>[2x]TRRTAFFFDELCLWHAAGPHALTLPVGGWVQPPAAAGHAESPETKRRLKSLLDVSGLTARLQLRSAPPASDEDLLRVHPAHYLERFKALSDAGGGSLGQDAPIGPGSYEIARLSAGLAIAALDAVLAGEADNAYSLSRPPGHHCLPDQAMGFCFFANIAVAIEAAKARHGVERVAVLDWDVHHGNGT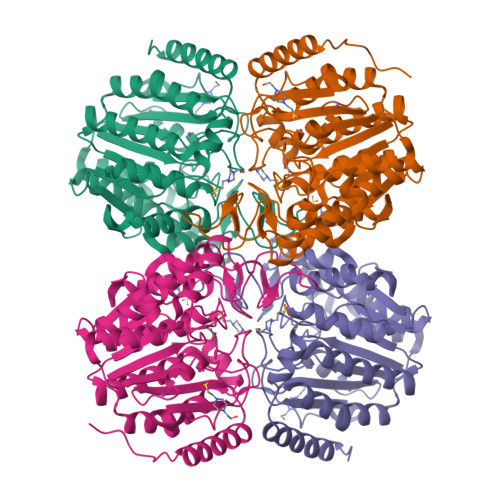QAIYYRRDDVLSISLHQDGCFPPGYSGAEDIGEDRGRGFNLNVPLLPGGGHDAYMQAMQRIVLPALERFRPQLIVVASGFDANAVDPLARMQLHSDSFRAMTAMVRDAAERHAGGRLVVVHEGGYSEAYVPFCGLAVIEELSGVRSAVRDPLRDFIELQQPNAAFRDFQRQRLEELAAQFGLCPAQPLQAAR>[3x]MSGESGQPEAGPSHAGLDWPNPERNRAGVPGGVIRRAGSQGPRSWIQKVLEQIMDSPRQCVTPSEVVPVTVLAVQRYLLEDEPRDTVPKPPLYCYDVTISDGVYQEKCYLDPSLNSLVYQNILKVGIQMRISRVSCLYNEKRIGQGILCIDNVHCGETSDSISLET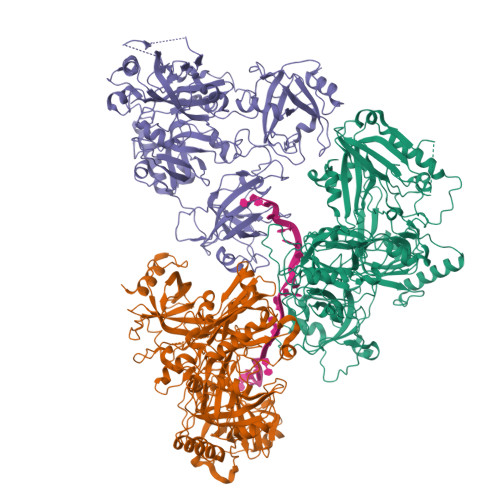PFRNRAHQEKPERPLRGGKSHYLALWNNEDPYGDIWLTDKQPEEHNFSDTKIISLSHLEMTWTNRRNFPALLVRILHKSKLRYYGKPDKKMIEPYQTFLEVADSSGTVSVIMWNALCPEWYKSLRVGLVLLLQDYSVKKSYPFRIQPVPVDPQIKLISTMEICLNLRDPPTNIIIIPEKQVKPEWRLPKLNHRFTTRSELDDMPENCICDVIGLLVFVGRVQRSKKKENREDFWSYRWIHIADGTSEQPFIVELFSTSQPEIFENIYPMAYFVCTQLKVVRNDNQVPKLLYLTTTNESGVFITGHRGQPYTYDAKVKNFIQWIRTKSDSGEQKNMVIGGYYPYPPVPETFSKYSSSIKVESLLTAISEVRKEIEDLQYREQKRIAIQGIITAIKYIPHSSATESASASETLRNANRPSTSQAARVEIQERNGKRHQDDEPVNSQYFQTTSTNLSLSNKIRILQGPHANPVAVPQPGASVQTKGIKPGMPSIFNRRANINANLQGKARKTISDRWESQLWREKKFGLIDHLHYSRVYPESIPRKFMFEHRKFLSDQYNSQPAKYVPPEGRPPKLDDFKSARSLGHFEVTILGLNHEIAIDVAFLPMYCPEDIRTSQIDTLLTSMNYSCAYPQDTTGNDRLPGPRAVAGDIIKAATELDRVHIVGILDICNLGNNKVEVYLHKIYSPENTS> GSHMQDPEQLKHCNGIL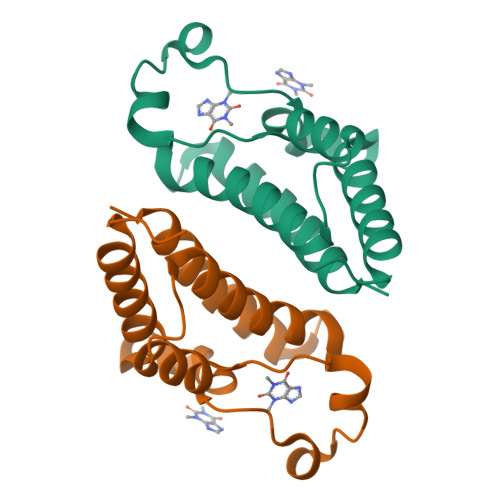KELLSKKHAAYAWPFYKPVDASALGLHDYHDIIKHPMDLSTVKRKMENRDYRDAQEFAADVRLMFSNCYKYNPPDHDVVAMARKLQDVFEFRYAKMPD> MTTTMKISIEFLEPFRMTKWQESTRRNKNNKEFVRGQAFARWHRNKKDNTKGRPYITGTLLRSAVIRSAENLLTLSDGKISEKTCCPGKFDTEDKDRLLQLRQRSTLRWTDKNPCPDNAETYCPFCELLGRSGNDGKKAEKKDWRFRIHFGNLSLPGKPDFDGPKAIGSQRVLNRVDFKSGKAHDFFKAYEVDHTRFPRFEGEITIDNKVSAEARKLLCDSLKFTDRLCGALCVIRFDEYTPAADSGKQTENVQAEPNANLAEKTAEQIISILDDNKKTEYTRLLADAIRSLRRSSKLVAGLPKDHDGKDDHYLWDIGKKKKDENSVTIRQILTTSADTKELKNAGKWREFCEKLGEALYLKSKDMSGGLKITRRILGDAEFHGKPDRLEKSRSVSIGSVLKETVVCGELVAKTPFFFGAIDEDAKQTALQVLLTPDNKYRLPRSAVRGILRRDLQTYFDSPCNAELGGRPCMCKTCRIMRGITVMDARSEYNAPPEIRHRTRINPFTGTVAEGALFNMEVAPEGIVFPFQLRYRGSEDGLPDALKTVLKWWAEGQAFMSGAASTGKGRFRMENAKYETLDLSDENQRNDYLKNWGWRDEKGLEELKKRLNSGLPEPGNYRDPKWHEINVSIEMASPFINGDPIRAAVDKRGTAVVTFVKYKAEGEEAKPVCAYKAESFRGVIRSAVARIHMEDGVPLTELTHSDCECLLCQIFGSEYEAGKIRFEDLVFESDPEPVTFDHVAIDRFTGGAADKKKFDDSPLPGSPARPLMLKGSFWIRRDVLEDEEYCKALGKALADVNNGLYPLGGKSAIGYGQVKSLGIKGDDKRISRLMNPAFDETDVAVPEKPKTDAEVRIEAEKVYYPHYFVEPHKKVEREEKPCGHQKFHEGRLTGKIRCKLITKTPLIVPDTSNDDFFRPADKEARKEKDEYHKSYAFFRLHKQIMIPGSELRGMVSSVYETVTNSCFRIFDETKRLSWRMDADHQNVLQDFLPGRVTADGKHIQKFSETARVPFYDKTQKHFDILDEQEIAGEKPVRMWVKRFIKRLSLVDPAKHPQKKQDNKWKRRKEGIATFIEQKNGSYYFNVVTNNGCTSFHLWHKPDNFDQEKLEGIQNGEKLDCWVRDSRYQKAFQEIPENDPDGWECKEGYLHVVGPSKVEFSDKKGDVINNFQGTLPSVPNDWKTIRTNDFKNRKRKNEPVFCCEDDKGNYYTMAKYCETFFFDLKENEEYEIPEKARIKYKELLRVYNNNPQAVPESVFQSRVARENVEKLKSGDLVYFKHNEKYVEDIVPVRISRTVDDRMIGKRMSADLRPCHGDWVEDGDLSALNAYPEKRLLLRHPKGLCPACRLFGTGSYKGRVRFGFASLENDPEWLIPGKNPGDPFHGGPVMLSLLERPRPTWSIPGSDNKFKVPGRKFYVHHHAWKTIKDGNHPTTGKAIEQSPNNRTVEALAGGNSFSFEIAFENLKEWELGLLIHSLQLEKGLAHKLGMAKSMGFGSVEIDVESVRLRKDWKQWRNGNSEIPNWLGKGFAKLKEWFRDELDFIENLKKLLWFPEGDQAPRVCYPMLRKKDDPNGNSGYEELKDGEFKKEDRQKKLTTPWTPWA;> MSNPIRDIQDRLKTAKFDNKDDMMNLASSLYKYEKQLMDSSEATLCQQGLSNRPNSFSQLSQFRDSDIQSKAGGQTGKFWQNEYEACKNFQTHKERRETLEQIIRFLQNGAEEKDADDLLLKTLARAYFHRGLLYRPKGFSVPARKVEAMKKAIAYCEIILDKNEEESEALRIWLYAAMELRRCGEEYPENFAEKLFYLANDGFISELYDIRLFLEYTEREEDNNFLDMILQENQDRERLFELCLYKARACFHLNQLNDVRIYGESAIDNAPGAFADPFWDELVEFIRMLRNKKSELWKEIAIKAWDKCREKEMKVGNNIYLSWYWARQRELYDLAFMAQDGIEKKTRIADSLKSRTTLRIQELNELRKDAHRKQNRRLEDKLDRIIEQENEARDGAYLRRNPPCFTGGKREEIPFARLPQNWIAVHFYLNELESHEGGKGGHALIYDPQKAEKDQWQDKSFDYKELHRKFLEWQENYILNEEGSADFLVTLCREIEKAMPFLFKSEVIPEDRPVLWIPHGFLHRLPLHAAMKSGNNSNIEIFWERHASRYLPAWHLFDPAPYSREESSTLLKNFEEYDFQNLENGEIEVYAPSSPKKVKEAIRENPAILLLLCHGEADMTNPFRSCLKLKNKDMTIFDLLTVEDVRLSGSRILLGACESDMVPPLEFSVDEHLSVSGAFLSHKAGEIVAGLWTVDSEKVDECYSYLVEEKDFLRNLQEWQMAETENFRSENDSSLFYKIAPFRIIGFPAE

Here, we determine the protein substrate, structure, and mechanism of a type III-E CRISPR-associated protease (CASP) from the marine anaerobe Desulfonema ishimotonii, reveal insight into its natural function in coordinating a transcriptional response to foreign genetic material, and engineer it for novel RNA sensing applications in vitro and in human cells. We identified that the largest protein, Csx30, is specifically cleaved in response to a target RNA. Csx29 consists of a three-helix bundle N-terminal domain (NTD), a TPR domain with eight repeats, and a protease region containing a pseudo-caspase (CHAT1) and active-caspase (CHAT2) domain that resembles separases. In both complexes, Cas7.2-Cas7.4 interface with the NTD, TPR and CHAT1 domains of Csx29.

By comparing the inactive and active complexes we observed a major structural change within the eighth repeat of the TPR domain, which we term the activation region (AR). The AR is bipartite, composed of AR1 (aa 313–325) and AR2 (aa 356–411), which stack with each other in the inactive state. For the inactive complex, 877,928 particles were extracted from 16,553 micrographs, and downscaled twofold. After cleaning poor quality particles by 3D classification (4 classes, tau_fudge = 4, 30 Å resolution reference, 25 iterations), remaining particles were subject to CTF refinement and Bayesian polishing, and one more round of 3D classification (4 classes, tau_fudge = 4, 15 Å resolution reference, 25 iterations, soft mask with 3 pixel hard edge, 8 pixel soft edge), and refinement, producing a reconstruction from 374,026 particles at 3.2-Å resolution. Since the peripheral regions of the complex, as well as Csx29 NTD, and the NTD-proximal parts within the TPR domain were flexible, focused refinement was performed to improve the EM density in those regions. After removing these particles, the remaining particles were focus-refined by performing local angular searches starting at 0.9 degree sampling, and using the classification mask, producing a reconstruction at 3.2-Å resolution.> FSGSEATAAILSRAPWSLQSVNPGLKTNSSGEPKFTKCRSPERETFSCH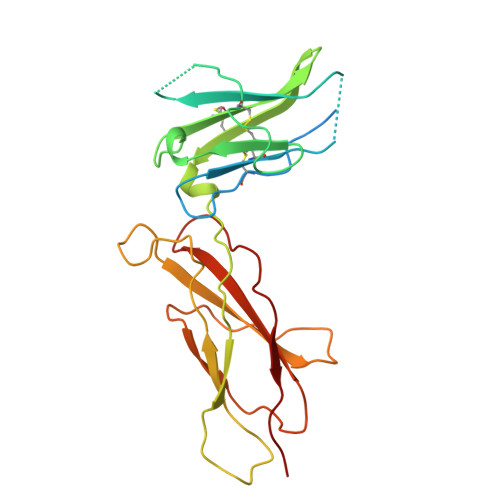WTDEVHHGTKNEGPIQLFYTRRNTQEWTQEWKECPDYVSAGENSCYFNSSFTSIAIPYCIKLTSNGGTVDEKCFSVDEIVQPDPPIALNWTLLNVSLTGIHADIQVRWEAPRNADIQKGWMVLEYELQYKEVNETKWKMMDPILTTSVPVYSLKVDKEYEVRVRSKQRNSGNYGEFSEVLYVTLPQM> MSGELSNRFQGGKAFGILKARQERRLAEINREFLCDQKYSDEENLPEKLTAFKEKYMEFDLNNEGEIDLMSLKRMMEKLGVPKTHLEMKKMISEVTGGVSDTISYRDFVNMMLGKRSAVLKLVMMFEGKANESSPKPVGPPPERDIASLP;>MSGELSNRFQGGKAFGLLKARQERRLAEINREFLCDQKYSDEENLPEKLTAFKEKYMEFDLNNEGEIDLMSLKRMMEKLGVPKTHLEMKKMISEVTGGVSDTISYRDFVNMMLGKRSAVLKLVMMFEG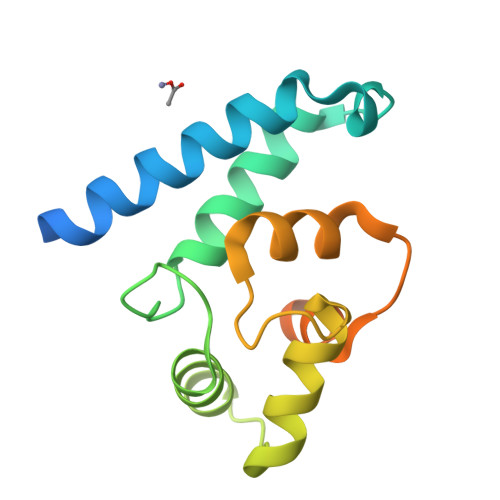KANESSPKPVGPPPERDIASLP[3x]> MNKQIFVLYFNIFLIFLGIGLVIPVLPVYLKDLGLTGSDLGLLVAAFALSQMIISPFGGTLADKLGKKLIICIGLILFSVSEFMFAVGHNFSVLMLSRVIGGMSAGMVMPGVTGLIADISPSHQKAKNFGYMSAIINSGFILGPGIGGFMAEVSHRMPFYFAGALGILAFIMSIVLIHDPKKSTTSGFQKLEPQLLTKINWKVFITPVILTLVLSFGLSAFQTLYSLYTADKVNYSPKDISIAITGGGIFGALFQIYFFDKFMKYFSELTFIA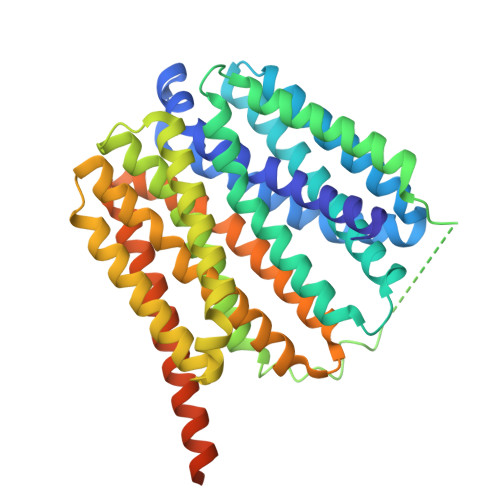WSLLYSVVVLILLVFANDYWSIMLISFVVFIGFDMIRPAITNYFSNIAGERQGFAGGLNSTFTSMGNFIGPLIAGALFDVHIEAPIYMAIGVSLAGVVIVLIEKQHRAKLKEQNMENLYFQGKLGPEQKLISEEDLNSAVDHHHHHHHHHH> MTAVVKNLAKLPAATSQILTNVSKLQTFHGLLEERRDKYAPLAYHTYDNLKQKTTWHPIAHAWVDEGLPVSKKEYNEYCWLKKDMQRLLPLASPFVFGIYGILPLAVWLSNDGYLPSAFSSKKDIVSKKLEWYSSYGDDLRQQVGPMLQH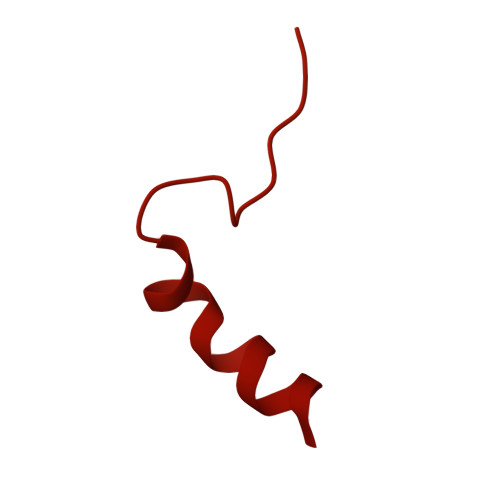RLKRHLRGTLNNEHRLMLDEVTESYKEIFYSHYTGQLRDVRKCAHLRLYDGTSTVLLLTNKEPVELTSELLQKWNAIKAAKLSPEEEKKARNEALIEAYKEQELHGGPHVKHMQGYGIPSDTPLLGENAKGDQYTQPPESASIPLEQLEWTGDTVFIPAEYRTEVEDWGRELTKLANQFLLLPWRFVSNAWNQRRLVSWFEEILQEDALIAKEGGVQALSDDELKVALLDRAVIRCDEELTRGDMEARYKEISWLMSLRNPFIVLAWQTGYYRSTYSPEDDLPEASILPKLNRTVLDVDVHNELAPDHPEKPLPRVHPALYPNSHLALAKEVAVLAK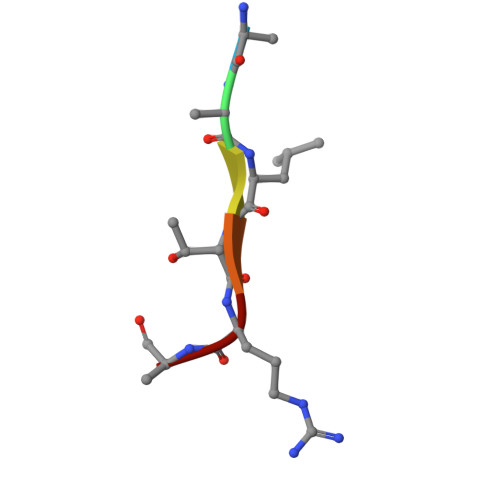> AALTRA5-ALPHA-ESTRAN-3,17-DIONE | C18 H26 O2 | 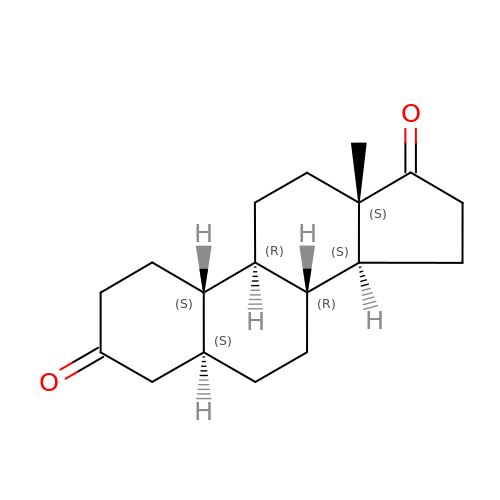CRDKSBHJIGNEOH-IMRIKWHGSA-N>[2x]MQKTLEVWIMPNSPQPAEDFKALVAPFEKAHGVEVKVTVLDWGVAWTKITTAATSGVGPDLTQLGTTWVGAISAMGVLEPVDDVLEALG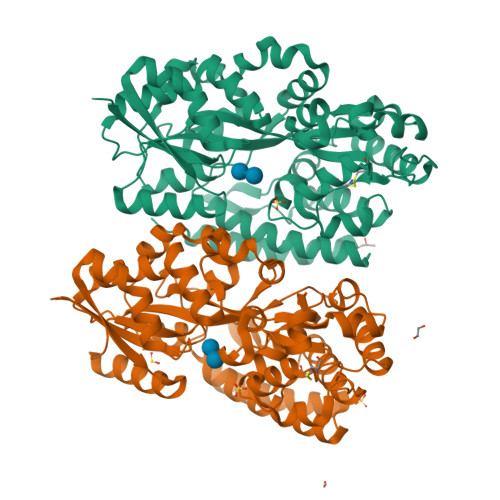GEKAYLPAVWRTTRLEGARQATAVPWFSELRAFYYRTDALKAAGVNPAEMFASWQGFEAGLARLKASSFRDPETKAPLAPLCTPGRTPRTLHNAAPWIWGAGGEIVRQAGGRWQSALNSPESLEGLYFFLSLAQKGYVPAESLEKNTAQIEADFQAGKCAVFASGPWMIQRAQVPEAKGGFAERTAAKNLGVAPYPAGPKGRYTFFGGSNLALFNFSKNKPLAKELLKYLGGPEAQVRYAQMTGMLPALRSAWSDPSFQQNPLLRTFIQAAQFGRTYPSLAGWGGVENLAVQHLGMAWDLVAQGRLTREALKDLMDKASAAINQALRHHHHHH> GPESAPRIMRLVAECSRSGARAGELRLPHGTVATPVFMPVGTQATMKGITTEQLDSLGCRICLGNTYHLGLRPGPELIRKAQGLHGFMNWPHNLLTDSGGFQMVSLFSLSEVTEEGVHFRSPYDGEETLLSPERSVEIQNALGSDIIMQLDHVVSSTVTGPLVEEAMHRSVRWLDR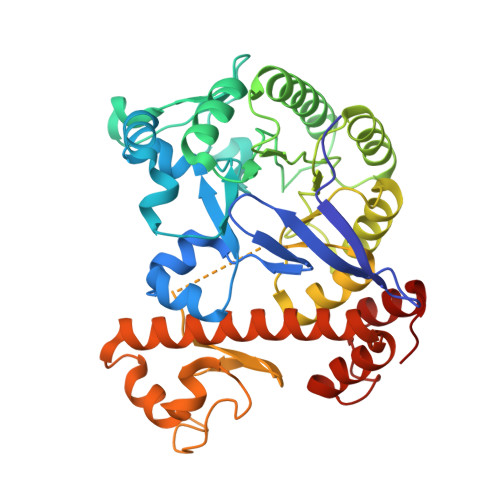CIAAHKHPDKQNLFAIIQGGLNADLRTTCLKEMTKRDVPGFAIGGLSGGESKAQFWKMVALSTSMLPKDKPRYLMGVGYATDLVVCVALGCDMFDCVYPTRTARFGSALVPTGNLQLKKKQYAKDFSPINPECPCPTCQTHSRAFLHALLHSDNTTALHHLTVHNIAYQLQLLSAVRSSILEQRFPDFVRNFMRTMYGDHSLCPAWAVEALASVGIMLT N-[2-(1H-benzimidazol-2-yl)ethyl]-2,2-dimethylpropanamide | C14 H19 N3 O | 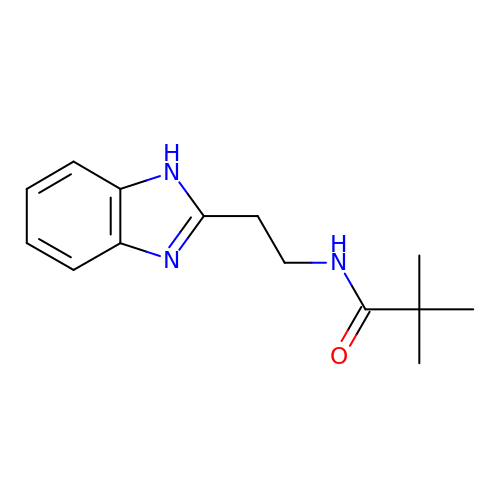UNNWFVAPBAIWDQ-UHFFFAOYSA-N> DNNIENIGDGAEVVKRTEDTSSDKWGVTQNIQFDFVKDKKYNKDALILKMQGFINSKTTYYNYKNTDHIKAMRWPFQYNIGLKTNDPNVDLINYLPKNKIDSVNVSQTLGYNIGGNFNSGPSTGGNGSFNYSKTISYNQQNYISEVERQNSKSVQWGIKANSFITSLGKMSG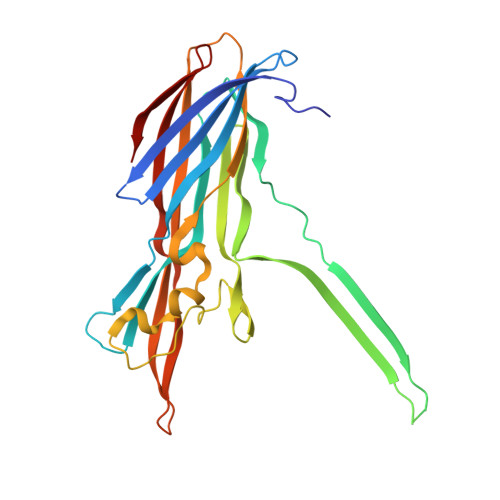HDPNLFVGYKPYSQNPRDYFVPDNELPPLVHSGFNPSFIATVSHEKGSGDTSEFEITYGRNMDVTHATRRTTHYGNSYLEGSRIHNAFVNRNYTVKYEVNWKTHEIKVKGHN>MRVNALLPLSGLIGTALAACPFADPSALGRRAEGGEVDARQRLKEVEVDDNGQFMTTDFGGNIEEQFSLKAGGRGSTLLEDFIFRQKLQHFDHERIPERVVHARGAGAHGIFTSYGDWSNITAASFLGAKDKQTPVFVRFSTVAGSRGSADTARDVHGFATRFYTDEGNFDIVGNNIPVFFIQDAIRFPDLIHSVKPSPDNEVPQAATAHDSAWDFFSSQPSALHTLFWAMSGNGIPRSYRHMDGFGIHTFRLVTEDGKSKLVKWHWKTKQGKAALVWEEAQVLAGKNADFHRQDLWDAIESGNAPSWELAVQLIDEDKAQAYGFDLLDPTKFLPEEFAPLQVLGEMTLNRNPMNYFAETEQISFQPGHIVRGVDFTEDPLLQGRLYSYLDTQLNRHRGPNFEQLPINRPVSGVHNNHRDGQGQAWIHKNIHHYSPSYLNKGYPAQANQTVGRGFFTTPGRTASGVLNRELSATFDDHYTQPRLFFNSLTPVEQQFVINAIRFEASHVTNEQVKKNVLEQLNKISNDVAKRVAVALGLEAPQPDPTYYHNNVTRGVSIFNESLPTIATLRVGVLSTTKGGSLDKAKALKEQLEKDGLKVTVIAEYLASGVDQTYSAADATAFDAVVVAEGAERVFSGKGAMSPL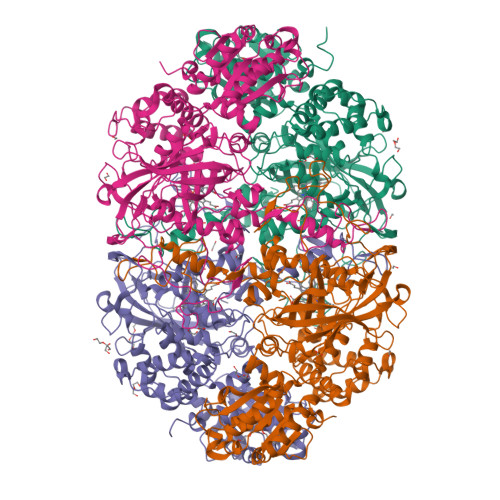FPAGRPSQILTDGYRWGKPVAAVGSAKKALQSIGVEEKEAGVYAGAQDEVIKGVEEGLKVFKFLERFAVDGDDEE[4x]> SNADVPIIDLQQDHLLIVQQITKACQDFGLFQVINHGVPEKLMVEAMEVYKEFFALPAEEKEKFQPKGEPAKFELPLEQKAKLYVEGERRCNEEFLYWKDTLAHGCYPLHEELLNSWPEKPPTYRDVIAKYSVEVRKLTMRILDYICEGLGLKLGYFDNELTQIQMLLANYYP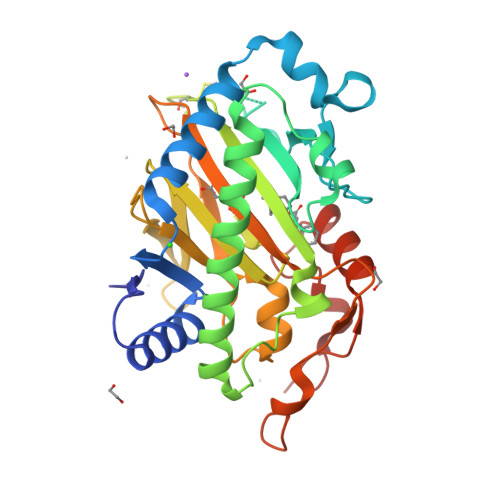SCPDPSTTIGSGGHYDGNLITLLQQDLVGLQQLIVKDDKWIAVEPIPTAFVVNLGLTLKVMSNEKFEGSIHRVVTHPIRNRISIGTLIGPDYSCTIEPIKELISQENPPLYKPYPYAEFAEIYLSDKSDYDAGVKPYKINQFPN[(1S)-1-(3,4-dichlorophenyl)-3-[oxidanyl-[2-[[3-(trifluoromethyl)phenyl]amino]phenyl]carbonyl-amino]propyl]phosphonic 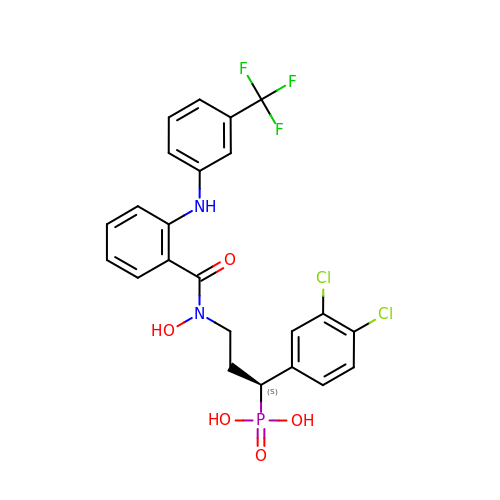acid | C23 H20 Cl2 F3 N2 O5 P | UCTDTGFTTGTERG-NRFANRHFSA-N>[4x]GGRPAGPRVTVLVREFEAFDNAVPELVDSFLQQDPAQPVVVAADTLPYPPLALPRIPNVRLALLQPALDRPAAASRPETYVATEFVALVPDGARAEAPGLLERMVEALRAGSARLVAAPVATANPARCLALNVSLREWTARYGAAPAAPRCDALDGDAVVLLRA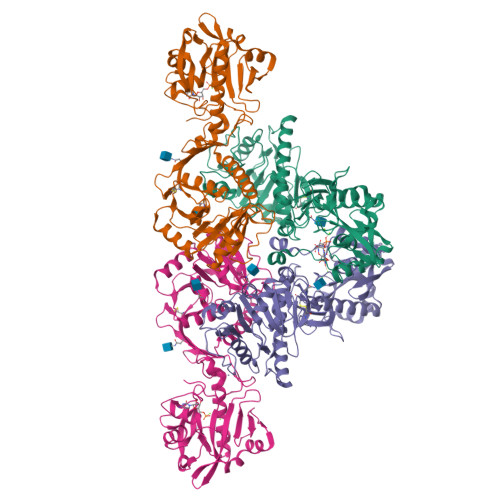RDLFNLSAPLARPVGTSLFLQTALRGWAVQLLDLTFAAARQPPLATAHARWKAEREGRARRAALLRALGIRLVSWEGGRLEWFGCNKETTRCFGTVVGDTPAYLYEERWTPPCCLRALRETARYVVGVLEAAGVRYWLEGGSLLGAARHGDIIPWDYDVDLGIYLEDVGNCEQLRGAEAGSVVDERGFVWEKAVEGDFFRVQYSESNHLHVDLWPFYPRNGVMTKDTWLDHRQDVEFPEHFLQPLVPLPFAGFVAQAPNNYRRFLELKFGPGVIENPQYPNPALLSLTGSG> 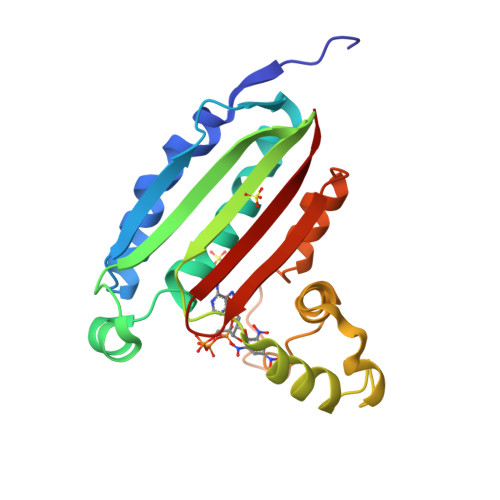VMKIRMVPISFVFNRFPRMVRDLAKKMNKEVNFIMRGEDTELDRTFVEEIGEPLLHLLRNAIDHGIEPKEERIAKGKPPIGTLILSARHEGNNVVIEVEDDGRGIDKEKIIRKAIEKGLIDESKAATLSDQEILNFLFVPGFSTKEKVSEVSGRGVGMDVVKNVVESLNGSISIESEKDKGTKVTIRLPLT In Drosophila melanogaster, Dicer-2 (DmDcr-2)-mediated RNAi pathway plays important roles in defending against viral infections and protecting genome integrity. During the maturation of siRNAs, two cofactors can regulate DmDcr-2’s functions: Loqs-PD that is required for dsRNA processing, and R2D2 that is essential for the subsequent loading of siRNAs into effector Ago2 to form RISC complexes. Here we present several cryo-EM structures of DmDcr-2/R2D2/Loqs-PD complex bound to dsRNAs with various lengths by the Helicase domain. These structures revealed that R2D2 and Loqs-PD can bind to different regions of DmDcr-2 without interfering with each other.

In order to investigate the effects on DmDcr-2’s function in the ternary complex during siRNA generation, we constructed the DmDcr-2 mutant (D1217N/D1476N, DmDcr-2DDNN) which exhibited no RNA dicing activity but possessed helicase activity in this work. To mimic the substrates and products, we designed and transcribed two dsRNAs, one with a length of 50 bp and the other with a length of 19 bp. From the 50-bp complex dataset, we acquired two structures: one in the dimer state with two DmDcr-2 molecules at a resolution of 3.72 Å, and another in the trimer state with three DmDcr-2 molecules at a resolution of 3.74 Å. In the dimer state structure, the model of dsRNA could be well fitted into the continuous density; however, compared with free dsRNA, we observed significant distortion. The 1st and 2nd DmDcr-2 are linked by this dsRNA, and there are large angles of tilt and twist between the two Helicase domains. This decoration pattern along dsRNA suggests that DmDcr-2’s Helicase domain can adopt a head-to-tail arrangement. Interestingly, when R2D2 was introduced into the same system, the arrangement of the two DmDcr-2 monomers transitioned to a head-to-tail configuration. This indicates that R2D2 plays a distinct role from Loqs-PD in the complex, as it can alter the aggregation mode of DmDcr-2. While dsRNA played a supportive role in the dimeric state, the DmDcr-2 monomers in the trimeric state exhibited much closer proximity to each other.

>MEDVEIKPRGYQLRLVDHLTKSNGIVYLPTGSGKTFVAILVLKRFSQDFDKPIESGGKRALFMCNTVELARQQAMAVRRCTNFKVGFYVGEQGVDDWTRGMWSDEIKKNQVLVGTAQVFLDMVTQTYVALSSLSVVIIDECHHGTGHHPFREFMRLFTIANQTKLPRVVGLTGVLIKGNEITNVATKLKELEITYRGNIITVSDTKEMENVMLYATKPTEVMVSFPHQEQVLTVTRLISAEIEKFYVSLDLMNIGVQPIRRSKSLQCLRDPSKKSFVKQLFNDFLYQMKEYGIYAASIAIISLIVEFDIKRRQAETLSVKLMHRTALTLCEKIRHLLVQKLQDMTYDDDDDNVNTEEVIMNFSTPKVQRFLMSLKVSFADKDPKDICCLVFVERRYTCKCIYGLLLNYIQSTPELRNVLTPQFMVGRNNISPDFESVLERKWQKSAIQQFRDGNANLMICSSVLEEGIDVQACNHVFILDPVKTFNMYVQSKGRARTTEAKFVLFTADKEREKTIQQIYQYRKAHNDIAEYLKDRVLEKTEPELYEIKGHFQDDIDPFTNENGAVLLPNNALAILHRYCQTIPTDAFGFVIPWFHVLQEDERDRIFGVSAKGKHVISINMPVNCMLRDTIYSDPMDNVKTAKISAAFKACKVLYSLGELNERFVPKTLKERVASIADVHFEHWNKYGDSVTATVNKADKSKDRTYKTECPLEFYDALPRVGEICYAYEIFLEPQFESCEYTEHMYLNLQTPRNYAILLRNKLPRLAEMPLFSNQGKLHVRVANAPLEVIIQNSEQLELLHQFHGMVFRDILKIWHPFFVLDRRSKENSYLVVPLILGAGEQKCFDWELMTNFRRLPQSHGSNVQQREQQPAPRPEDFEGKIVTQWYANYDKPMLVTKVHRELTPLSYMEKNQQDKTYYEFTMSKYGNRIGDVVHKDKFMIEVRDLTEQLTFYVHNRGKFNAKSKAKMKVILIPELCFNFNFPGDLWLKLIFLPSILNRMYFLLHAEALRKRFNTYLNLHLLPFNGTDYMPRPLEIDYSLKRNVDPLGNVIPTEDIEEPKSLLEPMPTKSIEASVANLEITEFENPWQKYMEPVDLSRNLLSTYPVELDYYYHFSVGNVCEMNEMDFEDKEYWAKNQFHMPTGNIYGNRTPAKTNANVPALMPSKPTVRGKVKPLLILQKTVSKEHITPAEQGEFLAAITASSAADVFDMERLEILGNSFLKLSATLYLASKYSDWNEGTLTEVKSKLVSNRNLLFCLIDADIPKTLNTIQFTPRYTWLPPGISLPHNVLALWRENPEFAKIIGPHNLRDLALGDEESLVKGNCSDINYNRFVEGCRANGQSFYAGADFSSEVNFCVGLVTIPNKVIADTLEALLGVIVKNYGLQHAFKMLEYFKICRADIDKPLTQLLNLELGGKKMRANVNTTEIDGFLINHYYLEKNLGYTFKDRRYLLQALTHPSYPTNRITGSYQELEFIGNAILDFLISAYIFENNTKMNPGALTDLRSALVNNTTLACICVRHRLHFFILAENAKLSEIISKFVNFQESQGHRVTNYVRILLEEADVQPTPLDLDDELDMTELPHANKCISQEAEKGVPPKGEFNMSTNVDVPKALGDVLEALIAAVYLDCRDLQRTWEVIFNLFEPELQEFTRKVPINHIRQLVEHKHAKPVFSSPIVEGETVMVSCQFTCMEKTIKVYGFGSNKDQAKLSAAKHALQQLSKCDA[2x];> MDQENFHGSSLPQQLQNLHIQPQQASPNPVQTGFAPRRHYNNLVGLGNGNAVSGSPVKGAPLGQRHVKLKKEKISAQVAQLSQPGQLQLSDVGDPALAGGSGLQGGVGLMGVILPSDEALKFVSETDANGLAMKTPVSILQELLSRRGITPGYELVQIEGAIHEPTFRFRVSFKDKDTPFTAMGAGRSKKEAKHAAARALIDKLIGAQLPESPSSSAGPSVTGLTVAGSGGDGNANATGGGDASDKTVGNPIGWLQEMCMQRRWPPPSYETETEVGLPHERLFTIACSILNYREMGKGKSKKIAKRLAAHRMWMRLQETPIDSGKISDSICGELEGEVSIIQDIDRYEQVSKDFEFIKI;>[2x]MDNKSAVSALQEFCARTQINLPTYSFIPGEDGGYVCKVELLEIEALGNGRSKRDAKHLAASNILRKIQLLPGIHGLMKDSTVGDLDEELTNLNRDMVKELRDYCVRREMPLPCIEVVQQSGTPSAPEFVACCSVASIVRYGKSDKKKDARQRAAIEMLALISSNSDNLRPDQMQVASTSKLKVVDMEESMEELEALRRKKFTTYWELKEAGSVDHTGMRLCDRHNYFKNFYPTLKKEAIEAINSDEYESSKDKAMDVMSSLKITPKISEVESSSLVPLLSVELNCAFDVVLMAKETDIYDHIIDYFRTMLI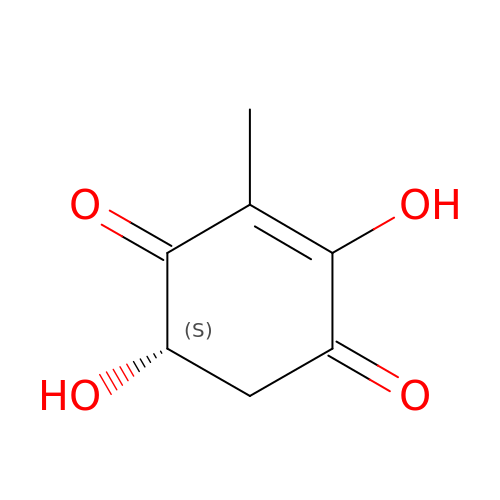(5S)-2,5-dihydroxy-3-methylcyclohex-2-ene-1,4-dione | C7 H8 O4 | CWBLUSPNRBEFNW-BYPYZUCNSA-N> MKVGINGFGRIGRQVFRILHERGVE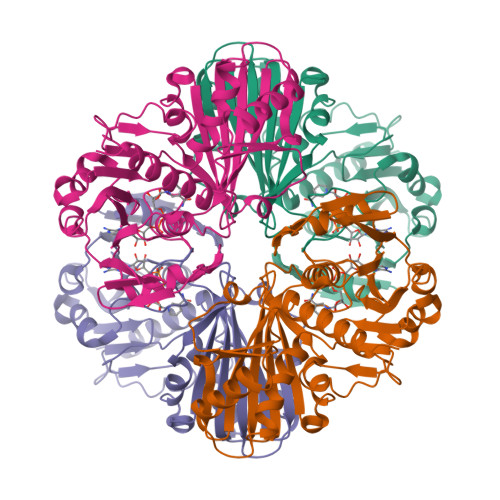VALINDLTDNKTLAHLLKYDSTYGRFPGAVGYDEENLYVDGKAIRATAIKDPREIPWKQAGVGVVVESTGVFTDGEKARAHLEAGAKKVIITAPAKNEDITVVLGVNHEQYDPAKHHILSNASCTTNSLAPVMKVLEKAFGVEKALMTTVHSYTNDQRLLDLPHKDLRRARAAALNIIPTTTGAAKATALVLPSLKGRFDGMALRVPTPTGSISDITALLKREVTAEEVNAALKAAAEGPLKGILAYTEDEIVLRDIVMDPHSSIVDGKLTKAIGNLVKVFAWYDNEWGYANRVADLVELVLKKGV> DYKDDDDKLHSQANLMRLKSDLFNRSPMYPGPTKDDPLTVTLGFTLQDIVKADSSTNEVDLVYYEQQRWKLNSLMWDPNEYGNITDFRTSAADIWTPDITAYSSTRPVQVLSPQ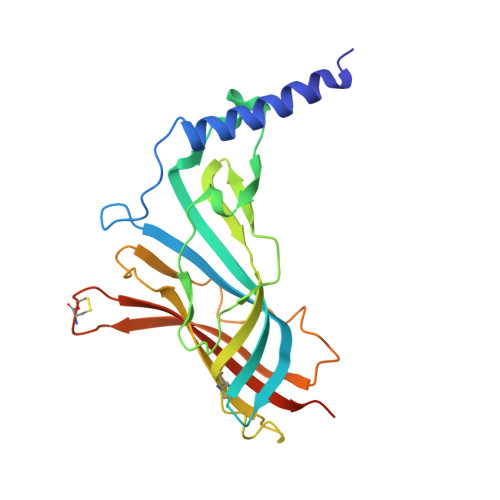IAVVTHDGSVMFIPAQRLSFMCDPTGVDSEEGATCAVKFGSWVYSGFEIDLKTDTDQVDLSSYYASSKYEILSATQTRQVQHYSCCPEPYIDVNLVVKFRERRAGNGFFRNLFD> SDKIIHLTDDSFDTDVLKADGAILVDFWAEWCGPSKMIAPILDEIADEYQGKLTVAKLNIDQNP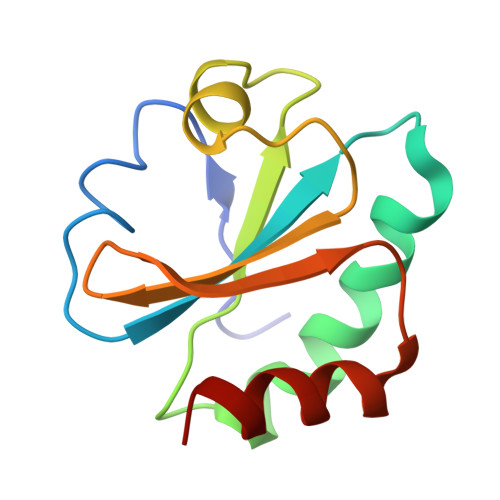GTAPKYGIRGIPTLLLFKNGEVAATKVGALSKGQLKEFLDANLA>[2x]MHRSPLAWLRLLLAAVLGAFLLGGPLHAAETAATRSPAWAQAVDPSINLYRMSPTLYRSALPNAQSVALLQRLQVKTVVSFIKDDDRAWLGQAPVRVLSLPTHADRVDDAEVLSVLRQLQAAEREGPVLMHCKHGNNRTGLFAAMYRIVVQGWDKQAALEEMQHGGFGDEDDMRDASAYVRGADVDGLRLAMANGECSPSRFAVCHVREWMAQALDRP

TpbA is a dual specific tyrosine phosphatase (DUSP) that has a conserved tyrosine phosphatase domain, and relevant phosphatase activities with p-nitrophenyl phosphate (pNPP) and phosphotyrosine peptides have been reported. TpbA (PA3885) from P. aeruginosa PA14 has been reported to be secreted to the periplasm and to link the extracellular quorum-sensing signals to EPS (extracellular polysaccharide) production and biofilm formation via negative regulation of c-di-GMP (3',5'-cyclic diguanylic acid), which regulates biological processes including motility and biofilm formation in bacteria. TpbA adopts a canonical eukaryotic-like DUSP fold with additional secondary structure elements that distinguish it from other DUSPs, including an N-terminal β-strand β0 that caps and extends the β-sheet, and a C-terminal helix α6 that packs on the outside of the protein. The active site architecture of the DUSP catalytic domain is defined by four loops: the protein tyrosine phosphatase (PTP) loop containing the conserved catalytic cysteine Cys132; the general acid loop containing a conserved aspartic acid that functions as a catalytic acid/base; a variable insert that varies among DUSPs and is predicted to involve in substrate recognition; and the α4-α5 loop that is equivalent to the Q-loop in protein tyrosine phosphatases (PTPs).

Native TpbA crystallises with two molecules in an asymmetric unit (a.s.u.), although our results and those of Koveal and colleagues show that it exists as a monomer in solution. The two molecules in an a.s.u. are continuously visible in the electron density map from residues 34–195 and have an identical conformation, yielding an r.m.s.d. of 0.1 Å for 161 aligned Cα atoms. In each TpbA monomer, additional electron density is observed adjacent to the PTP loop that is consistent with a phosphate ion that was introduced from the ammonium phosphate monobasic in the crystallization conditions. The phosphate binding is typical of DUSP enzymes, with main chain amide atoms in the active site PTP loop and the guanidine group from Arg138 strongly interacting with the oxygen atoms from the phosphate ion. The ligand-bound and the lowest energy ligand-free TpbA structures can be superimposed with an r.m.s.d. of 2.6 Å for 120 aligned residues, indicating significant conformational changes exist between the two structures. The core DUSP fold is essentially unchanged, but the largest structural changes occur in the PTP, general acid and α4-α5 loops, and at the C-terminal of the protein. The PTP loop, which binds phosphate, undergoes a maximum shift in Gly135 of 5.9 Å to accommodate the phosphate ion. The general acid loop, which is disengaged from the active site in the ligand-free state, becomes positioned close to the PTP loop via a 3.1 Å interaction between the backbone carbonyl of Thr102 and the conserved PTP arginine, Arg138.4-OXODECANEDIOIC 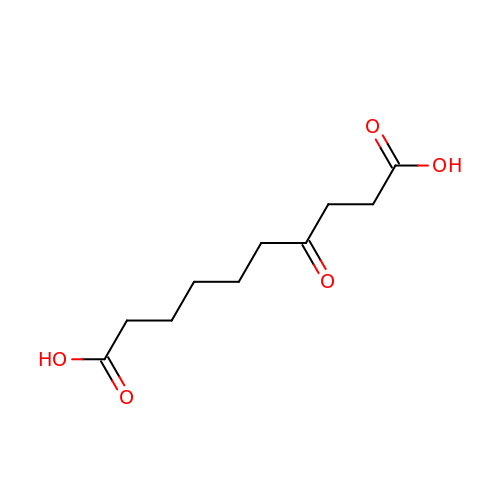ACID | C10 H16 O5 | XTQIBFVBYWIHIP-UHFFFAOYSA-N RdDM requires two plant-specific RNA polymerases known as RNA polymerase IV (Pol IV) and RNA polymerase V (Pol V), and a number of accessory proteins with different functions. All together, these observations have positioned the DDR complex as a key component that acts downstream of the methylation readers SUVH2/SUVH9 to recruit Pol V to RdDM loci. We report here the structures of the Arabidopsis Pol V recruitment complexes DR (DMS3-RDM1) and DDR′ (DRD1 peptide 7-DMS3-RDM1). The structures of the two complexes are similar at their core—two DMS3 dimers bridged by an RDM1 dimer.

When co-expressed in E. coli, DMS3, RDM1, and DRD1 peptide 7 formed a stable and isolatable complex that we called the DDR′ complex. Using single-particle cryoEM, we determined the structure of the DDR′ complex to an overall resolution of 3.5 Å. First, DRD1 peptide 7 forms three helices (α1, α2, and α3) and binds to DMS3-RDM1 in the DDR′ complex. Helix α1 is threaded into a symmetric, hydrophobic cleft formed by the RDM1 dimer interface involving the residues Lys121 and Leu128 (inset 1). On the other hand, α2 engages in hydrophobic interactions with two CC arms and one hinge from three DMS3 molecules, while α3 interacts with one CC arm and one hinge from two DMS3 molecules (inset 2). We attempted to model another DRD1 peptide 7 with the same interactions into the complex, however, this resulted in steric clashes between the two α1 helices. Therefore, the DDR′ complex most likely contains only one molecule of the peptide. A second major difference between the DR and DDR′ complexes is that the disordered CC arm of one DMS3h in the DR complex became ordered and visible in the DDR′ complex (i.e., the CC in DMS3hc2). Combined with the two DMS3 states already seen in the DR complex, we have three different DMS3 states (DMS3h, DMS3hc1 and DMS3hc2) in the DDR′ complex. The newly ordered CC arm is positioned close to the CC arm of DMS3hc1 from the same DMS3 dimer (DMS3hc1(E)-DMS3hc2(F)) in the DDR′ complex in a state that we refer as a “closed” state, and thus the corresponding DMS3 dimer which has a flexible CC arm in the DR complex is referred as an “open” state.

>[2x]MGSSHHHHHHSQDPSSMTMELRPSGDSGSSDVDAEISDGFSPLDTSHRDVADEGSLLRRAEMYQDYMKQVPIPTNRGSLIPFTSWVGLSISMKQLYGQPLHYLTNVLLQRWDQSRFGTDSEEQRLDSIIHPTKAEATIWLVEEIHRLTPSHLHMALLWRSDPMYHSFIDPIFPEK;>[4x]MADLYPTGQQISFQTTPLNVQDPTRMMNLDQSSPVARNETQNGGGIAHAEFAMFNSKRLESDLEAMGNKIKQHEDNLKFLKSQKNKMDEAIVDLQVHMSKLNSSPTPRSENSDNSLQGEDINAQILRHENSAAGVLSLVETLHGAQASQLMLTKGVVGVVAKLGKVNDENLSQILSNYLGTRSMLAVVCRNYESVTALEAYDNHGNIDINAGLHCLGSSIGREIGDSFDAICLENLRPYVGQHIADDLQRRLDLLKPKLPNGECPPGFLGFAVNMIQIDPAYLLCVTSYGYGLRETLFYNLFSRLQVYKTRADMISALPCISDGAVSLDGGIIRKTGIFNLGNRDEVNVRFAKPTASRTMDNYSEAEKKMKELKWKKEKTLEDIKREQVLREHAVFNFGKKKEEFVRCLAQSSCTNQPMNTPRGTLESGKETAAAKFERQHMDSSTSAA;> GEFFAVSNMLEALDSGKFGSVSKELEEIADMRMDLVKRSIWLYPSLAYTVFEAEKTMDGGGGSDYKDDDDK>MHHHHHHRTAGPKHVLLVSEHWDLFFQTKELLNPEEYRCTIGQQYKQELSADLVVCEYSLLPREIRSPKSLEGSFVLVLLDFFDEETSVDLLDRGFWYLI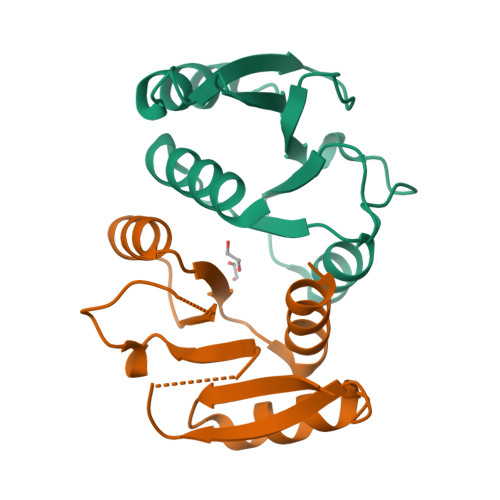RPITPRILKSAISLFLSQHSL[2x]> MGGKIYGEYLMLDKLLDAQCMLSEEDKRPVHDEHLFIITHQAYELWFKQIIFEFDSIRDMLDAEVIDETKTLEIVKRLNRVVLILKLLVDQVPILETMTPLDFMDFRKYLAPASGFQSLQFRLIENKLGVLTEQRVRYNQKYSDVFSDEEARNSIRNSEKDPSLLELVQRWLERTPGLEESGFNFWAKFQESVDRFLEAQVQSAMEEPVEKAKNYRLMDIEKRREVYRSIFDPAVHDALVRRGDRRFSHRALQGAIMITFYRDEPRFSQPHQLLTLLMDIDSLITKWRYNHVIMVQRMI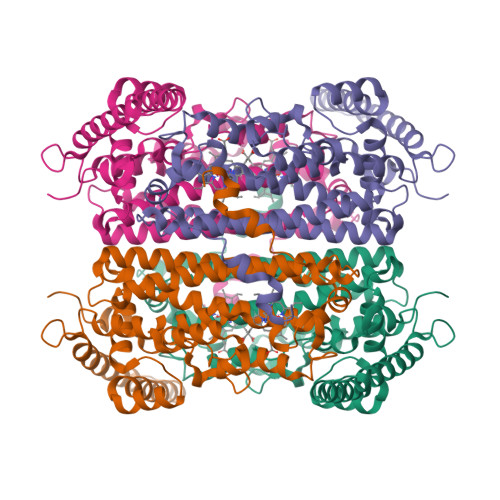GSQQLGTGGSSGYQYLRSTLSDRYKVFLDLFNLSTFLIPREAIPPLDETIRKKLINKSVLEHHHHHH> SQKVEKTVIKNETGTISISQLNKNVWVHTELGSFDGEAVPSNGLVLNTSKGLVLVDSSWDDKLTKELIEMVEKKFQKRVTDVIITHAHADRIGGIKTLKERGIKAHSTALTAELAKKNG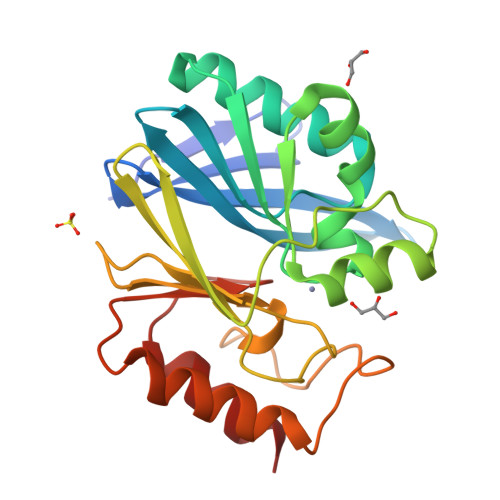YEEPLGDLQTVTNLKFGNMKVETFYPGKGHTEDNIVVWLPQYNILVGGCLVKSTSAKDLGNVADAYVNEWSTSIENVLKRYRNINAVVPGHGEVGDKGLLLHTLDLLK>SMFNSEIKEKYLDTLSEGMVMQMRPIFAKAEITETLYNKDIYDFTSMQILELIRSFDQTTIGSVRRTLALLSLYIDWAISYKLSKGLTNLARTISEEELYECLGDKKLYITYSELEEMENQLVNYQSKAVLRLLFEGVSGLAHSEL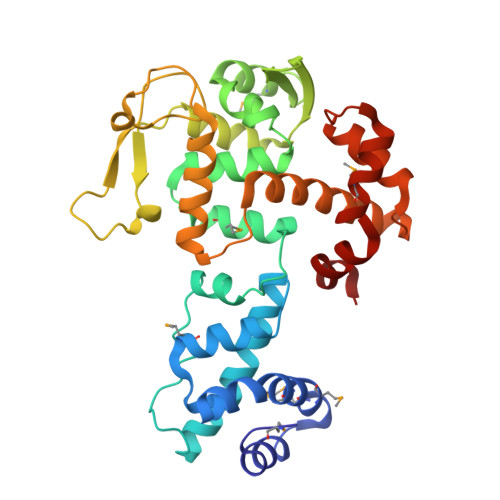LSLTKKQVEDAMLNGNVLTLYDSKHGERKLKVSSECLVIALNAAQETKYKLKNGKAKGQTKEVFLVENDYVVKTKRTSNKGDGQASKFVITNLITDISEFFKINFLTPNTIVRSGHLYRAYQLYKEKGVIDNSVRYQIIDDFNLRVKSKYRAVYSMQDYINEEEVNKYYAEELGL[3x]> AENSDFYLPGDYLLGGLFSLHANMKGIVHLNFLQVPMCKEYEVKVIGYNLMQAMRFAVEEINNDSSLLPGVLLGYEIVDVCYISNNVQPVLYFLAHEDNLLPIQEDYSNYSSRVVAVIGPDNSESVMTVANFLSLFLLPQITYSAISDELRDKVRFPALLRTTPSADHHIEAMVQLMLHFRWNWIIVLVSNDTYGRDNGQLLGERVARRGICIAFQETLPTLQPNQNMTSEERQRLVTIVDKLQQSTARVVVVFSPDLTLYHFFNEVLRQNFTGAVWIASESWAIDPVLHNLTELRHLGTFLGITIQSVPIPGFSEFREWGPQAGPPPLSRTSQSYTCNQECDNCLNATLSFNTILRLSGERVVYSVYSAVYAVAHALHSLLGCDKSTCTKRVVYPWQLLEEIWKVNFTLLDHQIFFDPQGDVALHLEIVQWQWDRSQNPFQSVASYYPLQRQLKNIQDISWHTINNTIPMSMCSKRCQSGQKKKPVGIHVCCFECIDCLPGTFLNHTEDEYE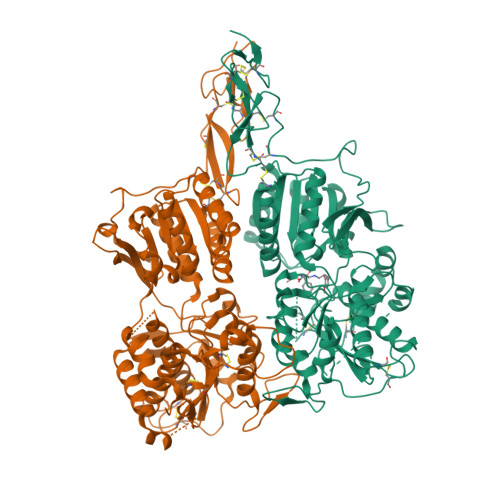CQACPNNEWSYQSETSCFKRQLVFLEWHEAPTIAVALLAALGFLSTLAILVIFWRHFQTPIVRSAGGPMCFLMLTLLLVAYMVVPVYVGPPKVSTCLCRQALFPLCFTICISCIAVRSFQIVCAFKMASRFPRAYSYWVRYQGPYVSMAFITVLKMVIVVIGMLATGLSPTTRTDPDDPKITIVSCNPNYRNSLLFNTSLDLLLSVVGFSFAYMGKELPTNYNEAKFITLSMTFYFTSSVSLCTFMSAYSGVLVTIVDLLVTVLNLLAISLGYFGPKCYMILFYPERNTPAYFNSMIQGYTMRRD;> ASLCLSQQFKAQGDYILGGLFPLGSTEEATLNQRTQPNSIPCNRFSPLGLFLAMAMKMAVEEINNGSALLPGLRLGYDLFDTCSEPVVTMKSSLMFLAKVGSQSIAAYCNYTQYQPRVLAVIGPHSSELALITGKFFSFFLMPQVSYSASMDRLSDRETFPSFFRTVPSDRVQLQAVVTLLQNFSWNWVAALGSDDDYGREGLSIFSSLANARGICIAHEGLVPQHDTSGQQLGKVLDVLRQVNQSKVQVVVLFASARAVYSLFSYSIHHGLSPKVWVASESWLTSDLVMTLPNIARVGTVLGFLQRGALLPEFSHYVETHLALAADPAFCASLNAELDLEEHVMGQRCPRCDDIMLQNLSSGLLQNLSAGQLHHQIFATYAAVYSVAQALHNTLQCNVSHCHVSEHVLPWQLLENMYNMSFHARDLTLQFDAEGNVDMEYDLKMWVWQSPTPVLHTVGTFNGTLQLQQSKMYWPGNQVPVSQCSRQCKDGQVRRVKGFHSCCYDCVDCKAGSYRKHPDDFTCTPCNQDQWSPEKSTACLPRRPKFLAWGEPVVLSLLLLLCLVLGLALAALGLSVHHWDSPLVQASGGSQFCFGLICLGLFCLSVLLFPGRPSSASCLAQQPMAHLPLTGCLSTLFLQAAETFVESELPLSWANWLCSYLRGLWAWLVVLLATFVEAALCAWYLIAFPPEVVTDWSVLPTEVLEHCHVRSWVSLGLVHITNAMLAFLCFLGTFLVQSQPGRYNRARGLTFAMLAYFITWVSFVPLLANVQVAYQPAVQMGAILVCALGILVTFHLPKCYVLLWLPKLNTQEFFLGRNAKKAADENSGGGEAAQGHNE>[2x]PGSPPGPPEDVKVEHISSTTSQLSWRPGPDNNSPIQIFTIQTRTPFSVGWQAVATVPEILNGQTYNATVVGLSPWVEYEFRVVAGNNIGIGEPSKPSELLRTKASVPNVAPGNINGGGGSRSELVITWEAIPEELQNGEGFGYIVMFRPVGTTAWMKERVALVESSKFIYRNESIMPLSPFEVKVGVY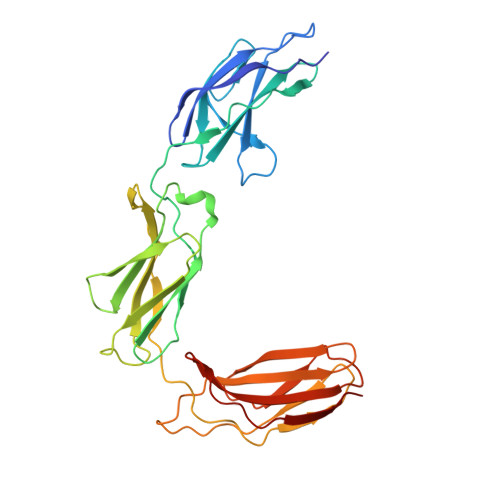NNEGEGSLSTVTIVYSGEDEPQLAPRGTSVQSFSASEMEVSWNAIAWNRNTGRVLGYEVLYWTDNSKESMIGKIRVSGNVTTKNITGLRANTIYFASVRAYNTAGTGPSSLPVNVTTKK MIF is a pleiotropic cytokine broadly studied in sepsis and many infectious and auto-immune diseases. Recently, a causative role in cancer progression has been attributed to MIF, as it has been reported to inactivate p53 (29), enhance angiogenesis, promote metastasis and impair both innate and adaptive immune responses. ISO-1, the ‘gold standard’ inhibitor of MIF, was designed to selectively ligate the tautomerase catalytic site of MIF which is known to neutralize its pro-inflammatory activity. We have identified ISO-66, a novel analog of ISO-1, as a potent inhibitor of MIF tautomerase activity.

To improve the solubility of ISO-66, the β-keto carboxylate was also synthesized (referred to as KF III 53Y/prodrug of ISO-66); however, it was found by mass spectrometry that KF III 53Y spontaneously decarboxylates to form ISO-66. This finding was also supported by structural studies, in which MIF was co-crystallized with KF III 53Y. ISO-66 was found bound in the MIF tautomerase active sites, with the meta-fluoro-para-hydroxyphenyl ring buried in the innermost part of the cleft, as expected. What was unexpected, however, was that the five-membered ring of the inhibitor had been opened. The bond between the nitrogen and oxygen was cleaved, resulting in free imine and hydroxyl groups. An open ring structure was seen in all three active sites. The hydroxyl group shares a hydrogen bond with Asn 97 at the base of the cavity. Lys 32 donates a strong hydrogen bond to the hydroxyl generated by the ring-opening reaction. The nitrogen that was formerly of the five-membered ring accepts a hydrogen bond from the main chain amide of Ile 64. In active site A, however, there was excess electron density around the methylene and terminal methyl ketone group of the inhibitor. It is very interesting that this excess density can be explained by the intact, ring-closed form of the inhibitor, having partial occupancy.

>[3x]PMFIVNTNVPRASVPDGFLSELTQQLAQATGKPPQYIAVHVVPDQLMAFGGSSEPCALCSLHSIGKIGGAQNRSYSKLLCGLLAERLRISPDRVYINYYDMNAANVGWNNSTFA> MPISPIETVPVKLKPGMDGPKVKQWPLTEEKIKALVEICTEMEKEGKISKIGPENPYNTPVFAIKKKDSTKWRKLVDFRELNKRTQDFWEVQLGIPHPAGLKQKKSVTVLDVGDAYFSVPLDKDFRKYTAFTIPSINNETPGIRYQYNVLPQGWKGSPAIFQCSMTKILEPFRKQNPDIVIYQYMDDLYVGSDLEIGQHRTKIEELRQHLLRWGFTTPDKKHQKEPPFLWMGYELHPDKWTVQPIVLPEKDSWTVNDIQKLVGKLNWASQIYAGIKVRQLCKLLRGTKALTEVVPLTEEAELELAENREILKEPVHGVYYDPSKDLIAEIQKQGQGQWTYQIYQEPFKNLKTGKYARMKGAHTNDVKQLTEAVQKIATESIVIWGKTPKFKLPIQKETWEAWWTEYWQATWIPEWEFVNTPPLVKLWYQLEKEPIIGAETFYVDGAANRETKLGKAGYV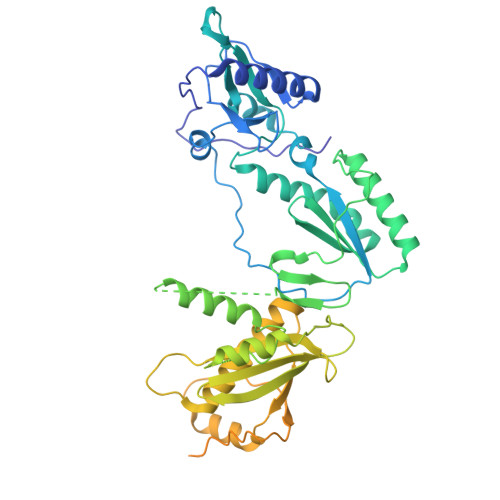TDRGRQKVVPLTDTTNQKTELQAIHLALQDSGLEVNIVTDSQYALGIIQAQPDKSESELVSQIIEQLIKKEKVYLAWVPAHKGIGGNEQVDGLVSAGIRKVLHHHHHHHHHH> NDPGKMLKDAIDKQAAGALVAGTSTSTHSVATDSTPALQAAETGATSTARDESMIETRTIVPTHGIHETSVESFFGRSSLVGMPLLATGTSITHWRIDFREFVQLRAKMSWFTYMRFDVEFTIIATSSTGQNVTTEQHTTYQVMYVPPGAPVPSNQDSFQWQSGCNPSVFADTDGPPAQFSVPFMSSANAYSTVYDGYARFMDTDPDRYGILPSNFLGFMYFRTLEDAAHQVRFRIYAKIKHTSCWIPRAPRQAPYKKRYNLVFSGDSDRICSNRASLTSY;> SPSAEACGYSDRVAQLTLGNSTITTQEAANICVAYGCWPAKLSDTDATSVDKPTEPGVSADRFYTLRSKPWQADSKGWYWKLPDALNNTGMFGQNAQFHYLYRGGWAVHVQCNATKFHQGTLLVLAIPEHQIATQEQPAFDRTMPGSEGGTFQEPFWLEDGTSLGNSLIYPHQWINLRTNNSATLILPYVNAIPMDSAIRHSNWTLAIIPVAPLKYAAETTPLVPITVTIAPMETEYNGLRRAIASNQ;> GLPTKPGPGSYQFMTTDEDCSPCILPDFQPTPEIFIPGKVNNLLEIAQVESILEANNREGVEGVERYVIPVSVQDALDAQIYALRLELGGSGPLSSSLLGTLAKHYTQWSGSVEITCMFTGTFMTTGKVLLAYTPPGGDMPRNREEAMLGTHVIWDFGLQSSITLVIPWISA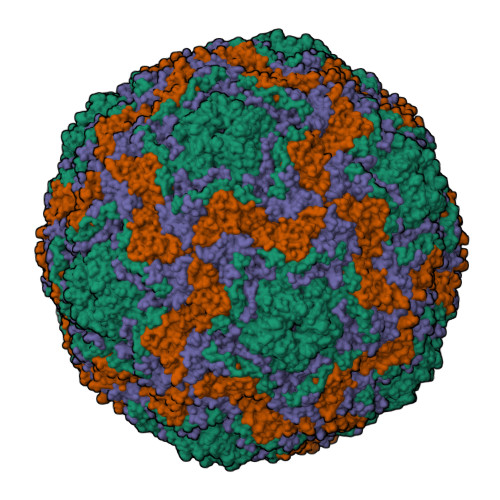SHFRGVSNDDVLNYQYYAAGHVTIWYQTNMVIPPGFPNTAGIIMMIAAQPNFSFRIQKDREDMTQTAILQ;> GAQLSRNTAGSHTTQTYATGGSTINYNNINYYSHAASAAQNKQDFTQDPSKFTQPIADVIKETAVPLK D-MYO-INOSITOL-1,4-BISPHOSPHATE | C6 H14 O12 P2 | 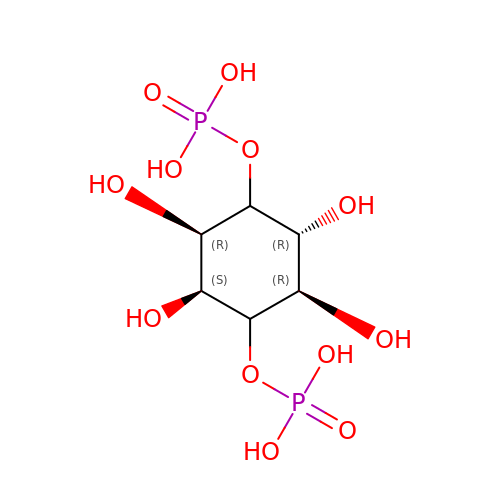PELZSPZCXGTUMR-GTTIYYRPSA-N> GDFVVVYTDGCCSSNGRRRPRAGIGVYWGPGHPLNVGIRLPGRQTNQRAE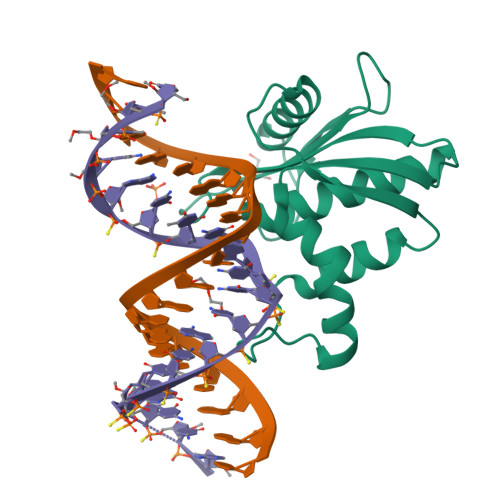IHAACKAIEQAKTQNINKLVLYTNSMFTINGITNWVQGWKKNGWKTSAGKEVINKEDFVALERLTQGMDIQWMHVPGHSGFIGNEEADRLAREGAKQSE>[4x]MAEYTLPDLDWDYGALEPHISGQINELHHSKHHATYVKGANDAVAKLEEARAKEDH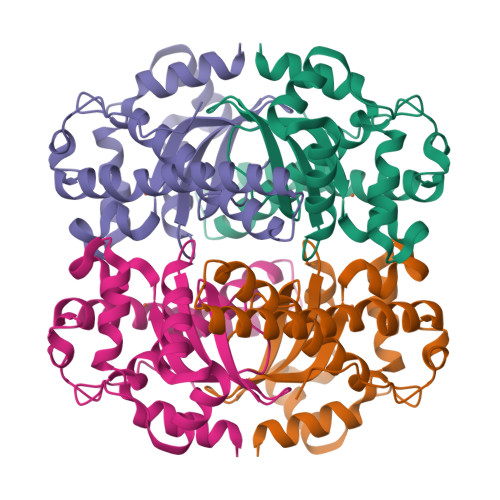SAILLNEKNLAFNLAGHVNHTIWWKNLSPNGGDKPTGELAAAIADAFGSFDKFRAQFHAAATTVQGSGWAALGWDTLGNKLLIFQVYDHQTNFPLAIVPLLLLDMWEHAFYLQYKNVKVDFAKAFWNVVNWADVQSRYAAATSQTKGLIFG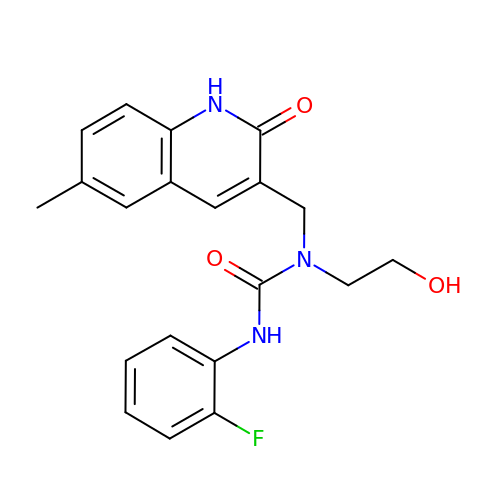3-(2-fluorophenyl)-1-(2-hydroxyethyl)-1-[(6-methyl-2-oxo-1,2-dihydroquinolin-3-yl)methyl]urea | C20 H20 F N3 O3 | IZEKTGGQNDYMPR-UHFFFAOYSA-N> MKYPPSLVSLIRELSRLPGIGPKSAQRLAFHLFEQPREDIERLASALLEAKRDLHVCPICFNITDAEKCDVCADPSRDQRTICVVEEPGDVIALERSGEYRGLYHVLHGVLSPMNGVGPDKLHIKPLLPRVGQGMEVILATGTTVEGDATALYLQRLLEPLGAAISRIAYGVP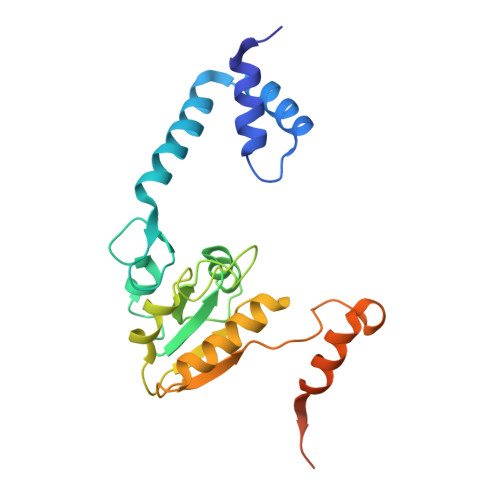VGGSLEYTDEVTLGRALTGRQTVSKPQPPQRPGDEDGADGAAVPASR The poly(ADP-ribose) polymerases (PARPs) Tankyrase (TNKS and ARTD5) and Tankyrase 2 (TNKS2 and ARTD6) regulate Wnt-β-catenin signaling (Huang et al., 2009). The two Tankyrases are highly similar (Hsiao and Smith, 2008, Smith et al., 1998), sharing a set of five ankyrin repeat clusters (ARCs) for substrate binding (Guettler et al., 2011, Seimiya et al., 2004), a sterile alpha motif (SAM) domain (De Rycker and Price, 2004, De Rycker et al., 2003), and a catalytic PARP domain (Rippmann et al., 2002). Tankyrase polymerization is mediated by the SAM domain, a small helical fold highly prevalent in eukaryotes (Knight et al., 2011, Qiao and Bowie, 2005). We report crystal structures of the polymerizing TNKS and TNKS2 sterile alpha motif (SAM) domains, revealing versatile head-to-tail interactions.

Since polymerization was likely to hinder crystallization, we used the polymerization-impaired DH902/924RET2 mutant. Reasoning that the mutant domain would still retain most polymerization interface residues, polymer contacts would be recoverable at the high protein concentration during crystallization, as illustrated for other polymerizing SAM domains (Kim et al., 2001, Kim et al., 2002). We obtained well-diffracting crystals (1.53 Å) and solved the structure by molecular replacement (Supplemental Experimental Procedures). The TNKS2 SAM domain, a 5-α-helix bundle similar to other SAM domains, formed a left-handed helix with a pitch of 46 Å, whose axis coincided with the crystallographic P65 screw axis. The SAM domains interacted in the well-established end-helix (EH)-mid-loop (ML) binding mode. On the EH surface, basic electrostatic potential predominated while the ML surface was predominantly acidic, in line with the salt sensitivity of the polymer. The closest approach between the two surfaces occurred around the N terminus of helix α5, where EH surface residues A919T2, Y920T2, G921T2, and H922T2 engaged in a network of hydrogen bonds and van der Waals contacts. Y920T2 was the most buried side chain at the interface (125 Å2), interacting with various hydrophobic ML side chains (V903T2, I899T2, I915T2, and M907T2), which collectively formed a shallow pocket, as well as E911T2 and E897T2. In its non-mutated form, D902T2 likely forms a salt bridge with R932T2, which may promote another salt bridge between K928T2 and E906T2. Surprisingly, despite its importance for TNKS2 SAM domain polymerization, R896T2 was not involved in any contact.

> SNAEKKEVPGVDFSITQFVRNLGLEHLMDIFEREQITLRVLVEMGHKELKEIGINAYGHREKLIKGVERLISGQQGL>[24x]MSTFPIDSGARIGEMKRVTKETNVSVKINLDGTGVADNSSGIPFLDHMLDQLASHGLFDVHVKATGDTHIDDHHTNEDVALAIGTAL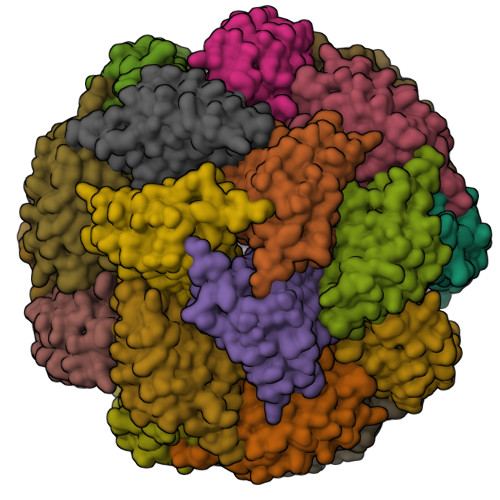LQALGDRKGINRFGNFSAPLDEALVHVSLDLSGRPHLGYDLNIPTQRVGKYDTQLVEHFFQSLVNTSGMTLHIRQFSGTNSHHIIEATFKAFARALRQATEYDTRRRGTIPSSKGVLSRS>GHMLLNSITELKGCARLFANIIEDEISEKLIVNYSDESIEDMKNHKTYKFTKLIQNFSHQNKDLFKEDLHVYIDFCLKRRENFNLFSVGSSNIPNTFEKLLAFFKNNYFDKFVITLQYVMLSDNADSQDLLSNNKDGGKDVEIKLKIEESTISLGSTLITLDEITDKLQIKKKYSQLNHQNGIGLSKFQFFCLQDIEPIPIDFYFIEIYQPSIYPILKRSTGTESNLNSPLEIVLKKIFHDTKSAFVFQIDHSAEVYDILKLSSHLSFIRNPKGK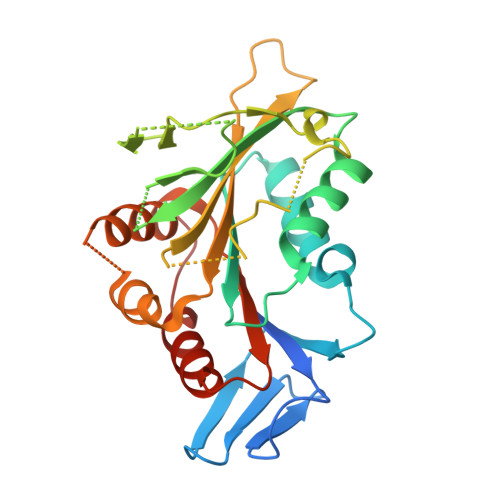[2x]> MAHHHHHHMEITAERWTYEVKDYLDTGMGIIRG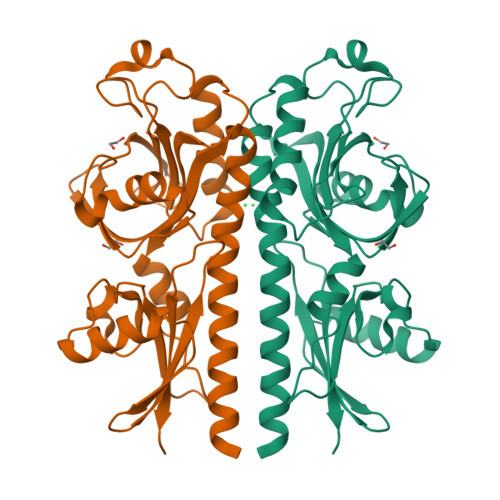FRFPLLFSAPPRNQIIAALREILKVNDHYFGARLAYEPNSLDGNDLEFQNTLGHDSTGRFIPYLHRGQTKEEIVLEDAKYYDSLGPEGDWYQVPKKTKSHYATDPYYYEIKGKVKILMMSLMVPLYVNDQFYGVAGLDYQLEELQQRIGVKKPFQDLGYLTLISPKGIYAVNGFDSNRVGEKISDAKELEYYLSKSQEGEKFTTDSDGYTHYYFPFHIGKDKRYWVMQVSIPNSIYKE Here, we show that a core component of the fork protection complex in the eukaryotic replisome, Timeless, harbours in its C‐terminal region a previously unappreciated DNA‐binding domain that exhibits specific binding to G‐quadruplex (G4) DNA structures. The FPC comprises four main proteins—Timeless, Tipin, Claspin and AND‐1—that are conserved from yeast to mammals. Inspection of the amino acid sequence of human Timeless revealed the presence of a conserved domain in its C‐terminal half (residues 816–954), with a predicted fold similarity to the myb‐like proteins of the homeodomain‐like superfamily, that bind double‐stranded DNA (dsDNA) with a tandem repeat of 3‐helix bundles (named here N‐term and C‐term). Our findings indicate that Timeless contributes to the ability of the replisome to sense replication‐hindering G4 formation and ensures the prompt resolution of these structures by DDX11 to maintain processive DNA synthesis.

We used X‐ray diffraction and NMR spectroscopy to investigate experimentally the structure and dynamics of the newly discovered Timeless domain. The 1.15 Å crystal structure of amino acids 885–947 (C‐term), corresponding to a single myb‐like fold, confirmed the presence of a three‐helix bundle characteristic of the homeodomain superfamily of DNA‐binding proteins, extended by the presence of a fourth C‐terminal alpha helix unique to the Timeless domain. The N‐ and C‐terminal domains adopted the same three‐dimensional fold; in particular, the N‐terminal repeat shared the presence of an additional fourth helix, H4, as seen in the C‐terminal repeat. A distinguishing feature of the Timeless DBD is the presence of a fourth alpha helix in both N‐ and C‐terminal 3‐helix bundle repeats. Superposition of the DBD C‐term onto the structurally homologous domains of the telomeric protein TRF1 (Court et al, 2005) and bacterial cell cycle regulator GcrA (Wu et al, 2018) in complex with their dsDNA substrates shows that, if the DBD were to adopt a similar mode of dsDNA binding, the fourth helix of both its N‐term and C‐term repeats would likely lead to a steric clash with the phosphate backbone of the DNA. Although it is conceivable that the DBD might rearrange its conformation upon DNA binding, the fourth helix of both repeats participates in core hydrophobic interactions, mediated by conserved residues L872 and F879 (N‐terminal repeat), and L936, V937 and L943 (C‐terminal repeat), making such rearrangements unlikely. We found that it bound with low micromolar affinity to both ss‐ and dsDNA probes. Indeed, when we tested a well‐characterised G4 sequence present in the promoter of the MYC gene (Ambrus et al, 2005), the DBD bound to it with nanomolar affinity, and about one order of magnitude tighter than ds‐ or ssDNA. While Timeless DBD binds to both ss‐ and dsDNA, it binds with ~ 10‐fold greater affinity to a defined G4 DNA sequence.

> DPGTHIVLWTGDQELELQRLFEEFRDSDDVLGHIMKNITAKRSRARIVDKLLALGLVAERRELYKKR>MTKIALIGSGQIGAIVGELCLLENLGDLILYDVVPGIPQGKALDLKHFSTILGVNRNILGTNQIEDIKDADIIVITAGVQRKEGMTREDLIGVNGKIMKSVAESVKLHCSKAFVICVSNPLDIMVNVFHKFSNLPHEKICGMAGILDTSRYCSLIADKLKVSAEDVNAVILGGHGDLMVPLQRYTSVNGVPLSEFVKKNMISQNEIQEIIQKTRNMGAEIIKLAKASAAFAPAAAITKMIKSYLYNENNLFTCAVYLNGHYNCSNLFVGSTAKINNKGAHPVEFPLTKEEQDLYTESIASVQSNT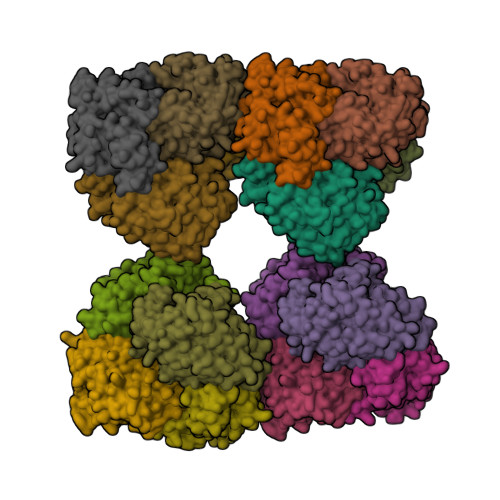QKAFDLIKGHHHHHH[16x]>[6x]GPLGSMKPINIQDQFLNQIRK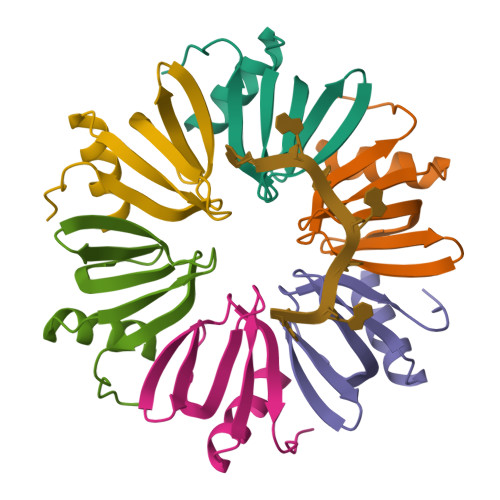ENTYVTVFLLNGFQLRGQVKGFDNFTVLLESEGKQQLIYKHAISTFAPQKNVQLELE> LKDSLRPKLSEEQQHIIAILLDAHHKTYDPTYADFRDFRPPVRMDGSTGSVTLDLSPLSMLPHLADLVSYSIQKVIGFAKMIPGFRDLTSDDQIVLLKSSAIEVIMLRSNQSFTMDDMSWDCGSQDYKYDVTDVSKAGHTLELIEPLIKFQVGLKKLNLHEEEHVLLMAICIVSPDRPGVQDAKLVEAIQDRLSNTLQTYIRCRHPPPGSHQLYAKMIQKLADL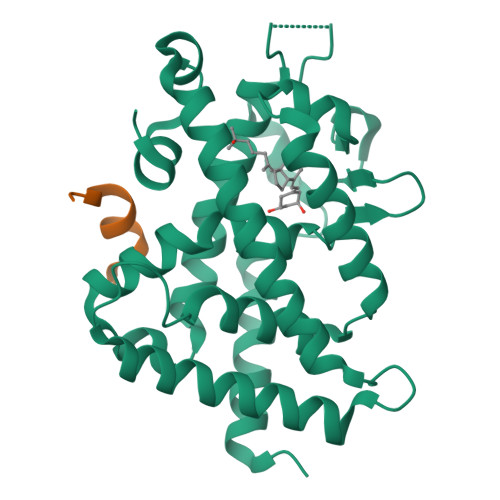RSLNEEHSKQYRSLSFQPENSMKLTPLVLEVFGNEISLVPRGSMAISDPNSSSVDKLAAALEHHHHHH;> KNHPMLMNLLKDN>MSD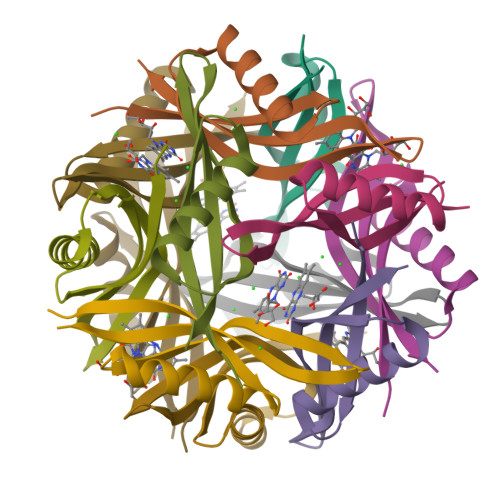HVYKIVELTGSSPNGIEEAVNNAIARAGETLRHLRWFEVVDTRGHIEGGRVNHWQVTVKVGFTLEGGLE[12x]> VPFFVNRGGLPVDEATWERMWKHVAKIHPDGEKVAQRIRGATDLPKIPIPSVPTFQPSTPVPERLEAVQRYIRELQYNHTGTQFFEIKK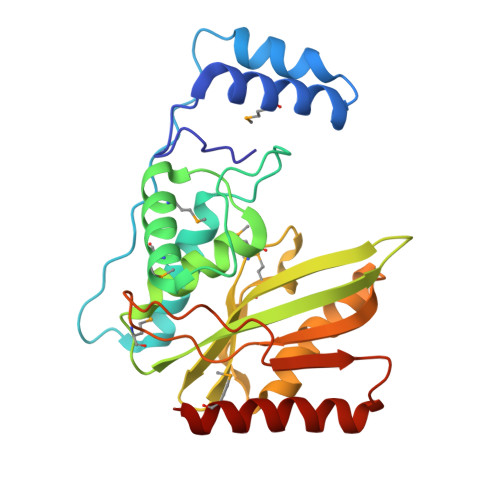SRPLTGLMDLAKEMTKEALPIKCLEAVILGIYLTNSMPTLERFPISFKTYFSGNYFRHIVLGVNFAGRYGALGMSRREDLMYKPPAFRTLSELVLDFEAAYGRCWHVLKKVKLGQSVSHDPHSVEQIEWKHSVLDVERLGRDDFRKELERHARDMRLKI>[3x]MAGGDDLKLLGAWPSPFVTRVKLAL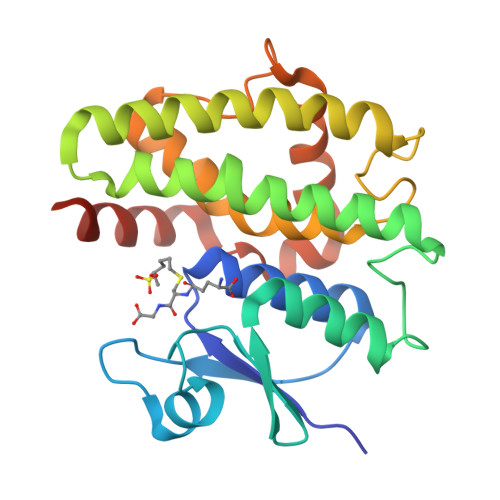ALKGLSYEDVEEDLYKKSELLLKSNPVHKKIPVLIHNGAPVCESMIILQYIDEVFASTGPSLLPADPYERAIARFWVAYVDDKLVAPWRQWLRGKTEEEKSEGKKQAFAAVGVLEGALRECSKGGGFFGGDGVGLVDVALGGVLSWMKVTEALSGDKIFDAAKTPLLAAWVERFIELDAAKAALPDVGRLLEFAKAREAAAAASK>MAKQFLYDNLPVVETKAGKLRGYQWEGTYIFKGIRYARANRFQLPEEVEPWEGVKEAASYGFVCPMLTRDHPQGELLVPHRYWPQDEDCLSLNIWSQSLDRSAKKPVMFWIHGGAFSMGSSIEQKAYNGENMS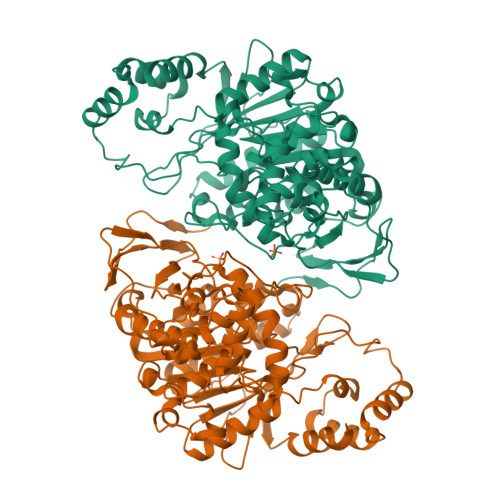RYGDVVVVTVNHRLNILGYLDLSPYGERYAGSANAGQADLVAALKWVRDNIEAFGGDPDNVTIFGQSGGGMKVSGLMQTPEADGLFHRAMIMSGVAGDVLPYSTGDSRPLIQAMLKELGLAEQEAGRLETVPYYDLAAAYNRVSPAIARAGGYIGCTPRPDDFYKGEGPAVGFTDHAKTIPVMVGTVFGEFAMMPLPFNKETISEAELDEILDKRFQGHGKELKTVFAEAYPGKSPVDLLTLDTIFRGPTKEFVRSLAAAGGSVYSYLFALEFPYQNQKTAWHCSDIPFIFHNTELVPVTNIPEISDKLEKQMFDAVIHFVETGDPNHLGIPQWPVSTEDREATMIFDRVCTVRFNFDDYLLELYKKALPNLTLANITQEDNQIQHALE[4x]2-[butyl(oxidanyl)-$l^{3}-sulfanyl]-4-(2,3-dimethylimidazol-4-yl)-6-(1,3-thiazol-2-yl)thieno[2,3-b]pyridin-3-amine | C19 H23 N5 O S3 | 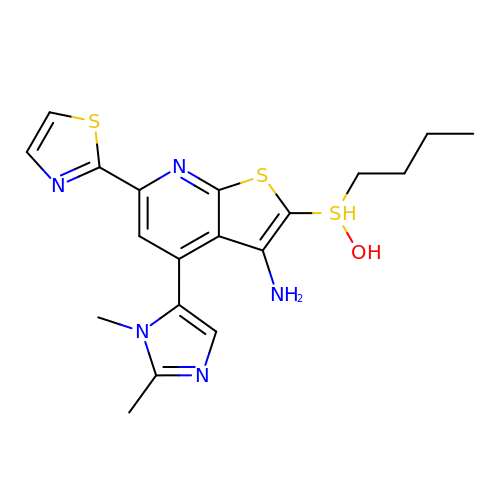UNHFBUMWCMKPAQ-UHFFFAOYSA-N>MRIFGYARVSTSQQSLDIQIRALKDAGVKANRIFTDKASGSSTDREGLDLL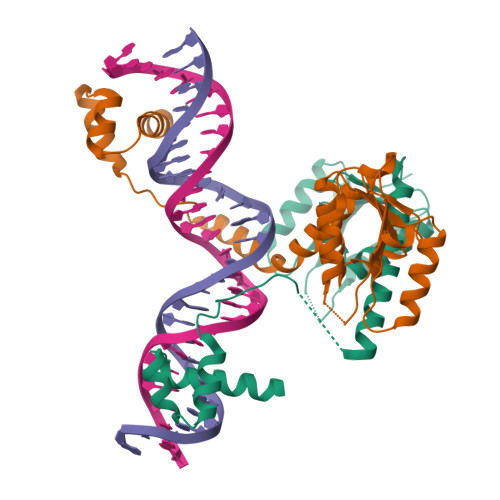RMKVEEGDVILVKKLDRLGRDTADMIQLIKEFDAQGVAVRFIDDGISTDGDMGQMVVTILSAVAQAERRRILERTNEGRQEAKLKGIKFGRRRTVDRNVVLTLHQKGTGATEIAHQLSIARSTVYKILEDERASAHHHHHH[4x]>MAHHHHHHMDLGIAG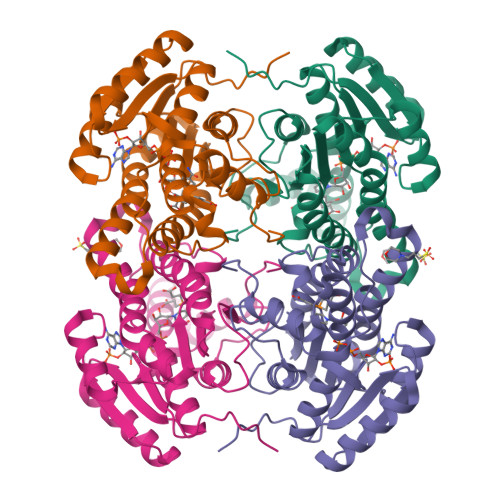KSALVCAASKGLGRGCAEALAAEGVNVTIVARTPETLDATAAAIRANAGVDVQAVACDITTPEGRAAALAACPQPDILVNNAGGPPPGDFRNFTHDDWIRALEANMLTPIELIRATIDGMISRGFGRVVNITSSSVKAPIDVLGLSNGARSGLTGFIAGVARKVAPNGVTINNLLPGIFDTDRIAVTFDAAAKAQNISVDEARKQRMATIPARRFGTPDEFGRACAFLCSVHAGYITGQNWLIDGGAYPGTY[4x]Apoptosis-inducing factor mitochondrial 1 (AIFM1) is a NADH-binding flavin adenine dinucleotide (FAD)-dependent oxidoreductase in the mitochondrial intermembrane space (IMS). It plays key roles in mitochondrial function, respiratory chain maintenance, redox control, and non-caspase-dependent cell death. Upon NADH binding, an air-stable FADH2-NAD+ charge-transfer complex (CTC) forms, inducing AIFM1 dimerization and the release of a C-terminal regulatory segment termed C-loop. We solved three structures of human soluble AIFM1 (aa 103–613) by cryo-EM: the dimer (1) without interactors (termed “AIFM1 dimer”), (2) bound to AK2A, or (3) to MIA40.

We obtained reconstructions for the AIFM1 dimer and AIFM1-AK2A and AIFM-MIA40 complexes at global resolutions of 2.8, 2.6, and 2.4 Å, respectively. We built atomic models of AIFM1 aa 128–611 (lacking aa 511–557 [AIFM1 dimer or AIFM1-MIA40] or aa 511–549 [AIFM1-AK2A] due to flexibility), as well as the interacting residues 232–239 of AK2A and 2–20 of MIA40, into these maps. All our structures resemble reduced AIFM1, i.e., NAD+ bound after CTC formation. Consequently, we observe the hallmark re-orientation conformation of the “aromatic tunnel” side chains (F310, Y347, W351, F482, Y492, F508, Y560, and W579) connecting the central cofactors and periphery of the C-terminal domain26. Concurrently, a loop connecting two C-terminal β-strands (aa 487–489) releases W198 of the so-called β-clasp that is part of the regulatory β-hairpin (aa 190–202). Consequently, the C-loop is released, providing surface accessibility to the binding site of electron acceptors or a second NADH cofactor. The AIFM1 dimer and, in particular, AIFM1-MIA40 show inter-protomer variability predominantly of NAD binding and parts of the C-terminal domain, whereas little displacement was seen when comparing AK2A-bound protomers. The inter-protomer variability of AIFM1 within the AIFM1 dimer and AIFM1-MIA40 suggests structural asymmetry within the complex. This is also reflected in the variability of local cryo-EM densities of the sixth β-strand of AIFM1 added to the C-terminal β-sheet in the dimer, as well as in reported inter-protomer differences within the dimer. Although NADH leads to rapid AIFM1 dimerization, dimers dissociated with a half-life (t1/2) of ∼4 h upon removal of excess NADH.

>[2x]MASMTGGQQMGRGSEFMGGLTPEQKQKKAALSASEGEEVPQDKAPSHVPFLLIGGGTAAFAAARSIRARDPGARVLIVSEDPELPYMRPPLSKELWFSDDPNVTKTLRFKQWNGKERSIYFQPPSFYVSAQDLPHIENGGVAVLTGKKVVQLDVRDNMVKLNDGSQITYEKCLIATGGTPRSLSAIDRAGAEVKSRTTLFRKIGDFRSLEKISREVKSITIIGGGFLGSELACALGRKARALGTEVIQLFPEKGNMGKILPEYLSNWTMEKVRREGVKVMPNAIVQSVGVSSGKLLIKLKDGRKVETDHIVAAVGLEPNVELAKTGGLEIDSDFGGFRVNAELQARSNIWVAGDAACFYDIKLGRRRVEHHDHAVVSGRLAGENMTGAAKPYWHQSMFWSDLGPDVGYEAIGLVDSSLPTVGVFAKATAQDNPKSATEQSGTGIRSESETESEASEITIPPSTPAVPQAPVQGEDYGKGVIFYLRDKVVVGIVLWNIFNRMPIARKIIKDGEQHEDLNEVAKLFNIHEDAAALEHHHHHH> TEETSITNFYSRAGLVGVVNMPVQGTSNTKGFAKWGIDIMGFVQMRRKLELMTYMR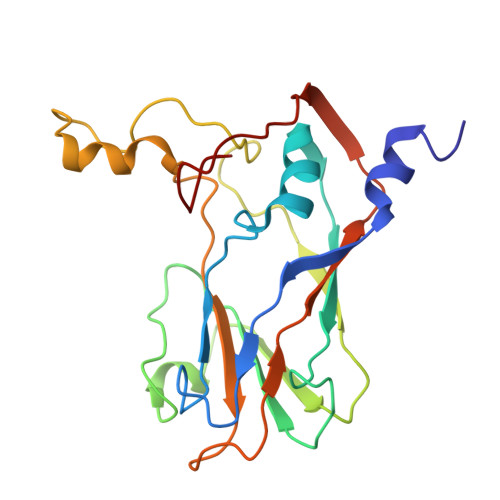FSAEFTFVASTPEGETTNLILQYMYAPPGAPLPTRRDSYEWQTSTNPSIISKMADPPAQVSVPFLSPASAYQWFYDGYPTFGKHPIDQDFQYGMCPNNMMGTFCVRMIGGGKPTQSVTIRIYMRLKHIRAWVPRPLRSQNYTMRNYPN>GSSGSSGPTYPKYLLSPETIEALRKPTFDVWLWEPNEMLSCLEHMYHDLGLVRDFSINPVTLRRWLFCVHDNYRNNPFHNFRHCFCVAQMMYSMVWLCSLQEKFSQTDILILMTAAICHDLDHPGYNNTYQINARTELAVRYNDISPLENHHCAVAFQILAEPECNIFSNIPPDGFKQIRQGMITLILATDMARHAEIMDSFKEKMENFDYSNEEHMTLLKMILIKCCDISNEVRPMEVAEPWVDCLLEEYFMQSDREKSEGLPVAPFMDRDKVTKATAQIGFIKFVLIPMFETVTKLFPMVEEIMLQ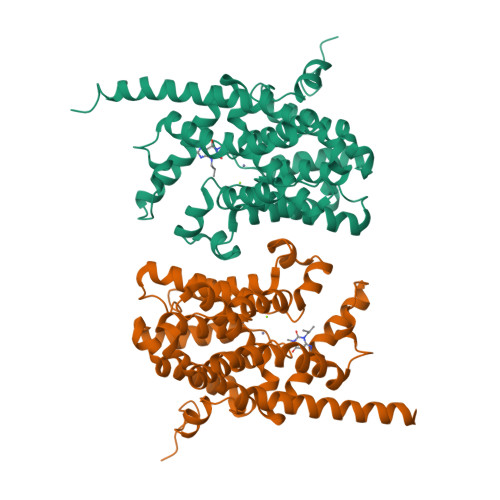PLWESRDRYEELKRIDDAMKELQKK[2x]> SHMASMKKKGSVVIVGRINLSGDTAYAQQTRGEEGCQETSQTGRDKNQVEGEVQIVSTATQTFLAT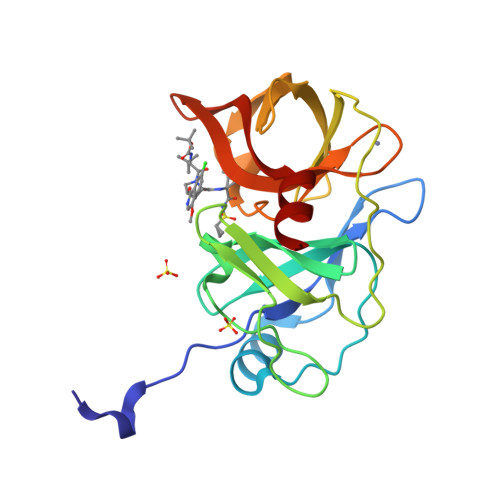SINGVLWTVYHGAGTRTIASPKGPVTQMYTNVDKDLVGWQAPQGSRSLTPCTCGSSDLYLVTRHADVIPVRRRGDSRGSLLSPRPISYLKGSSGGPLLCPAGHAVGIFKAAVSTRGVAKAVDFIPVESLETTMR> MSGHGNLEEMEATDGFSFRTLFRRYRTPLTAAATLIVFCLVGYAIMQLTNEVRYDDVVAALAATGPSAILLALFFTALSFLSLVFYDLNAIEYIGKKLPFPHVALTAFSAYAVGNTAGFGALSGGAIRYRAYTRLGLSPEDIGRIIAFVTLSFGLGLAAVASIALIIIASEIGPLIGVSPFLLRLIAGSIIAILGAVM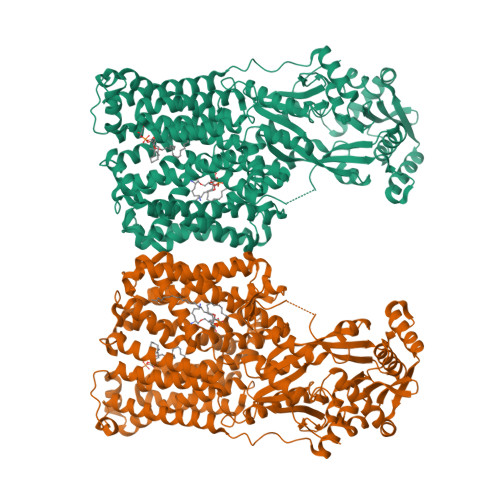IIGREGRVLNFGAVAIRLPDSRTWSRQFLVTAFDIAASASVLYVLLPQTAIGWPVFLAVYAIAVGLGVLSHVPAGLGVFETVIIASLGSAVNIDAVLGSLVLYRLIYHVLPLLIAVLAVSAAELRRFVDHPAASSVRRIGGRLMPQLLSTLALLLGVMLVFSSVTPTPDQNLEFLSNYLPLPMVEGAHFLSSLLGLALVVAARGLGQRLDGAWWVAVFSAVAALTLSLLKAIALVEAAFLAFLIFGLFVSRRLFTRHASLLNQAMTASWLMAIAVIVVGAVVILLFVYRDVEYSNELWWQFEFTAEAPRGLRALLGITIISSAIAIFSLLRPATFRPEPATEEALTRAVEIVRKQGNADANLVRMGDKSIMFSEKGDAFIMYGRQGRSWIALFDPVGDHGAVQELVWRFVEAARAAGCRAVFYQISPALLSHCADAGLRAFKLGELAVADLRTFEMKGGKWANLRQTASRAQRDGLEFAVVEPENVPDIIDELAAVSTAWLEHHNAKEKGFSLGSFDPDYVSAQPVGILKKDGKIVAFANILVTESKEEGTIDLMRFSPDAPKGSMDFLFVQIMEYLRNQGFTHFNLGMAPLSGMSKREAAPVWDRIGSTVFEHGERFYNFKGLRAFKSKFHPHWQPRYLAVSGGGNPMIALMDATFLIGGGLKGVVRK> APSTDHLDYKDDDDKAAAKVFLCPGLLKGVYQSEHLFESDHQSGAWCKDPLQASDKIYYMPWTPYRTDTLTEYSSKDDFIAGRPTTTYKLPHRVDGTGFVVYDGALFFNKERTRNIVKFDLRTRIKSGEAIIANANYHDTSPYRWGGKSDIDLAVDENGLWVIYATEQNNGKIVISQLNPYTLRIEGTWDTAYDKRSASNAFMICGILYVVKSVYEDDDNEATGNKIDYIYNTDQSKDSLVDVPFPNSYQYIAAVDYNPRDNLLYVWNNYHVVKYSLDFGPLDSRSGPVHHG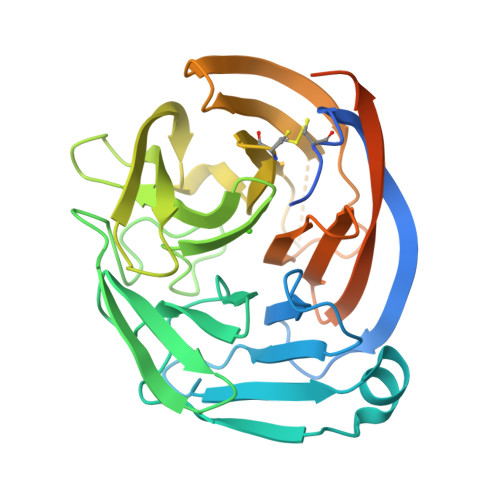QVSYISPPIHLDSELERPPVRGILEVLFQ>[2x]MALSKQYIPDDMELIFHMDGNVNGHYFTIVATGKAKPYEGKQNLKATVTKGAPLPFSTDILSTVMHYGNRCIVHYPPGIPDYFKQSFPEGYSWERTFAFEDGGFCTVSADIKLKDNCFIHTSMFHGTNFPADGPVMQRKTIQWEKSIEKMTVSDGIVKGDITMFLLLEGGGKYRCQFHTSYKAKKVVEMPQSHYVEHSIERTNDDGTQFELNEHAVARLNEILEHHHHHH

Wild-type SAASoti and its monomeric variant mSAASoti can undergo phototransformations, including reversible photoswitching of the green form to a nonfluorescent state and irreversible green-to-red photoconversion. Photoswitchable, photoconvertible and multi-transformable proteins are fine tools for multimodal measurements using super-resolution microscopy. Reversible photoswitching often proceeds via the cis–trans isomerization of the chromophore, associated with the change in its protonation state and plane distortions of the π-conjugated system. Photoconversion is an irreversible photochemical process of peptide chain breaking, leading to the formation of a new π-conjugated system and a redshift of the spectral parameters.

As it was shown in the previous study, C21N substitution abolished a dimeric fraction of the mSAASoti at higher concentrations and resulted in the true monomeric protein. The crystal structure of the C21N mSAASoti variant in its green on-state was obtained at 3.0 Å resolution. The analysis of crystal contacts demonstrated that SAASoti is a monomer supporting biochemical data. The mSAASoti has a typical β-barrel fold with the chromophore 66HYG68 resided on the central α-helix. In spite of the moderate resolution, the electron density clearly revealed a maturated chromophore in its cis-conformation as well as conformation of nearby residues. The chromophore is fixed with a number of hydrogen bonds with neighboring amino acid residues. The oxygen of the chromophore carbonyl group is hydrogen bonded to side chain of H120, while oxygen of imidazolidone moiety is fixed with side chain of two arginine residues—R70 and R95. Histidine group of the chromophore forms hydrogen bond to side chain of Q42. Finally, the OH-group of the tyrosine moiety is hydrogen bounded to side chain of S146. Noteworthy, the orientation of the chromophore’s tyrosine ring is stabilized through stacking interaction with side chain of H197.> MHHHHHHSSGRENLYFQGMGEKLELRLKSPVGAEPAVYPWPLPVYDKHHDAAHEIIETIRWVCEEIPDLKLAMENYVLIDYDTKSFESMQRLCDKYNRAIDSIHQLWKGTTQPMKLNTRPSTGLLRHILQQVYNHSVTDPEKLNNYEPFSPEVYGETSFDLVAQMIDEIKMTDDDLFVDLGSGVGQVVLQVAAATNCKHHYGVEKADIPAKYAETMDREFRKWMKWYGKKHAEYTLERGDFLSEEWRERIANTSVIFVNNFAFGPEVDHQLKERFANMKEGGRIVSSKPFAPLNFRINSRNLSDIGTIMRVVELSPLKGSVSWTGKPVSYYLHTIDRTILENYFSSLKNPKLREEQEAARRRQQRESKSNAATPTKGPEGKVAGPADAPMDSGAEEEKAGAATVKKPSPSKARKKKLNKKGRKMAGRKRGRPK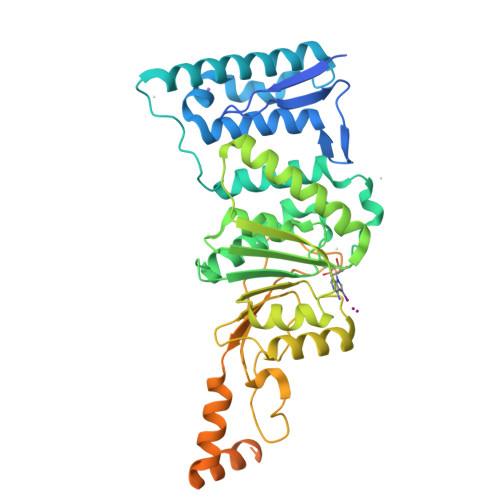KMNTA>[2x]AAPSFDCGKPQVEPK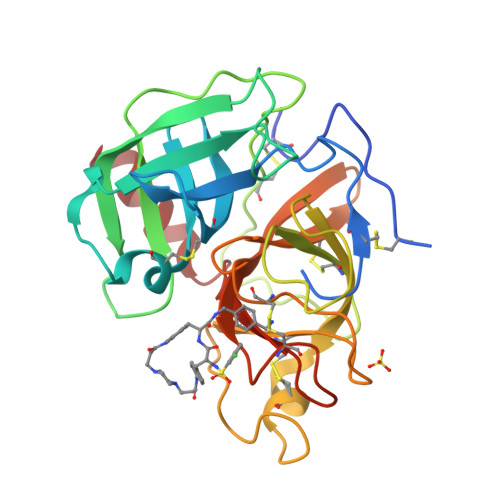KCPGRVVGGCVAHPHSWPWQVSLRTRFGMHFCGGTLISPEWVLTAAHCLEKSPRPSSYKVILGAHQEVNLEPHVQEIEVSRLFLEPTRKDIALLKLSSPAVITDKVIPACLPSPNYVVADRTECFITGWGETQGTFGAGLLKEAQLPVIENKVCNRYEFLNGRVQSTELCAGHLAGGTDSCQGDAGGPLVCFEKDKYILQGVTSWGLGCARPNKPGVYVRVSRFVTWIEGVMRNN> MKKLIPILEKIPEVELPVKEITFKEKLKWTGIVLVLYFIMGCIDVYTAGAQIPAIFEFWGRIGTLITLGIGPIVTAGIIMQLLVGSGIIQMDLSIPENRALFQGCQKLLSIIMCFVEAVLFVGAGAFGILTPLLAFLVIIQIAFGSIILIYLDEIVSKYGIGSGIGLFIAAGVSQTIFVGALGPEGYLWKFLNSLIQGVPNIEYIAPIIGTIIVFLMVVYAECMRVEIPLAHGRIKGAVGKYPIKFVYVSNIPVIL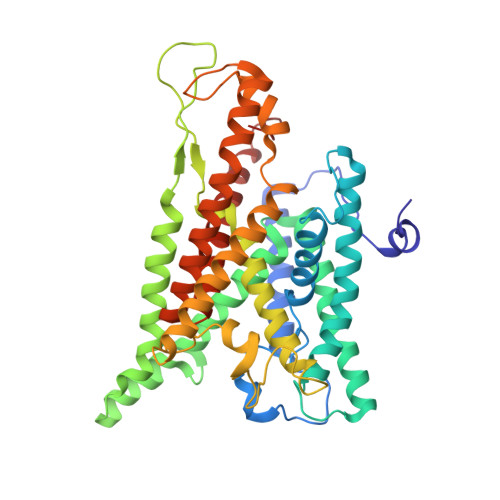AAALFANIQLWGLALYRMGIPILGHYEGGRAVDGIAYYLSTPYGLSSVISDPIHAIVYMIAMIITCVMFGIFWVETTGLDPKSMAKRIGSLGMAIKGFRKSEKAIEHRLKRYIPPLTVMSSAFVGFLATIANFIGALGGGTGVLLTVSIVYRMYEQLLREKVSELHPAIAKLLNK> AQPDIKFASKEYGVTIGESRIIYPLDAAGVMVSVKNTQDYPVLIQSRIYDENKEKESEDPFVVTPPLFRLDAKQQNSLRIAQAGGVFPRDKESLKWLCVKGIPPKDEDIWVDDATNKQKFNPDKDVGVFVQFAINNCIKLLVRPNELKGTPIQFAENL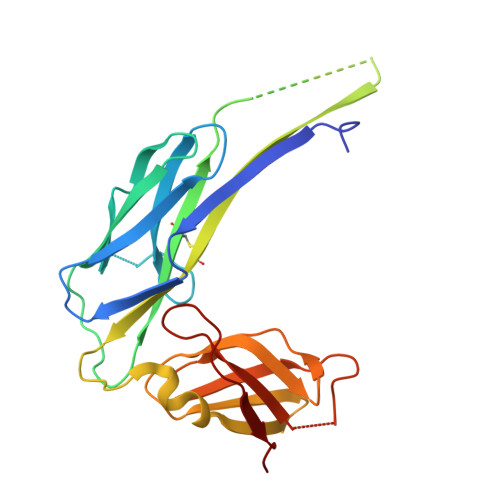SWKVDGGKLIAENPSPFYMNIGELTFGGKSIPSHYIPPKSTWAFDLPKGLAGARNVSWRIINDQGGLDRLYSKNVTL>GYMLGS[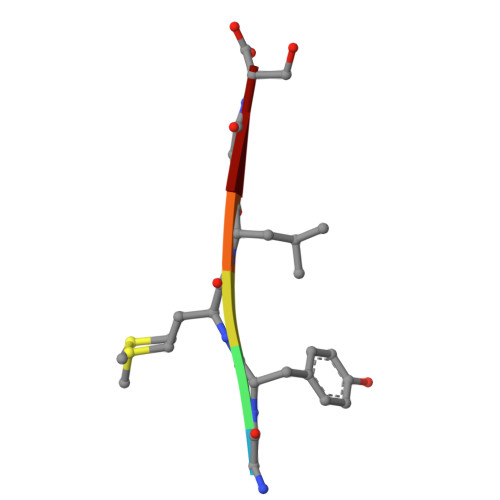2x]Histamine-Releasing Factor (HRF), also referred to as Translationally Controlled Tumour Protein (TCTP), p21, p23 and fortilin, is ubiquitously expressed in eukaryotes, and involved in apoptosis, cell cycle progression, cell proliferation and cancer (Bommer and Thiele, 2004, Nagano-Ito and Ichikawa, 2012, Bommer, 2012). In addition to its diverse range of intracellular roles, HRF is also able to activate mast cells and basophils, with the release of histamine (MacDonald et al., 1995, Kashiwakura et al., 2012), implicating a role in allergic disease. HRF can form dimers (Yoon et al., 2000; Kim et al., 2009, Kashiwakura et al., 2012), and a disulphide-linked dimer was shown to be crucial for the cytokine-like activity of rat HRF. mHRF, hHRF and rat HRF contain two cysteine residues, at positions 28 and 172, and Cys172 is suggested to be the site of the intermolecular disulphide bond. The current model for the activity of HRF in mast cell activation involves cross-linking of FcεRI-bound IgE by dimeric HRF, mediated by interactions between HRF and the Fab regions of IgE.

We report here the first crystal structure of murine HRF (mHRF), solved at 4.0 Å resolution, revealing the conserved HRF fold. The structure of mHRF was solved at 4.0 Å resolution, and contains two molecules in the asymmetric unit. Residues 1–38 and 68–170, and 1–41 and 67–170 were modeled for chains A and B, respectively; similar to other crystal structures of HRF (Vedadi et al., 2007, Susini et al., 2008, Dong et al., 2009, Eichhorn et al., 2013), the mobile loop region (residues Thr39-Val66) was disordered. mHRF contains a C-terminal His-tag, which was also disordered; a substantial region of continuous electron density was observed close to the C-terminus, but the tag could not be modeled with certainty.Fig. 1 mHRF. The overall fold of mHRF is conserved, and comprises three α-helices packed against two β-sheets, while a third β-sheet forms the base of the mobile loop. Like hHRF, mHRF contains two cysteine residues at positions 28 and 172, and thus has the potential to form a covalently-linked dimer; while Cys28 is buried, Cys172 is surface exposed. However, the two molecules of the mHRF asymmetric unit, which are related by non-crystallographic two-fold symmetry, form only non-covalent interactions. The two molecules bury a surface area of 176 Å2 at their interface, in which Glu80-Thr84 from one chain pack against equivalent residues from the other, with a hydrogen bond between Ser82 from each chain. Furthermore, the human and murine proteins are 96% identical, and the residues involved in forming both the disulphide bond and dimer interface are identical.

>MIIYRDLISHDELFSDIYKIREIADGLCLEVEGKMVSRTEGAIDDSLIGGNASAEGPEGEGTESTVVTGVDIVMNHHLQETSFTKEAYKKYIKDYMKSLKGKLEEQKPERVKPFMTGAAEQIKHILANFNNYQFFIGENMNPDGMVALLDYREDGVTPFMIFFKDGLEMEKCLEHHHHHH[2x]>[2x]MSLPMLQVALDNQTM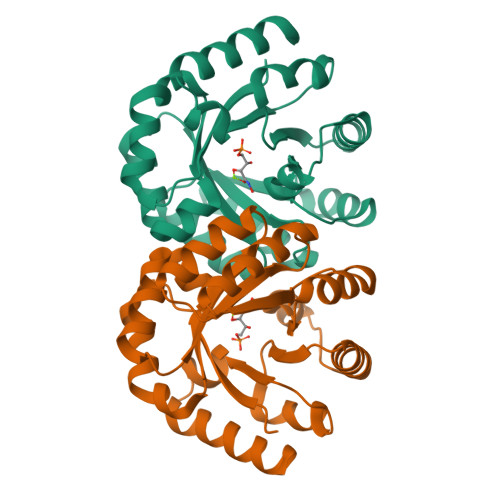DSAYETTRLIAEEVDIIEVGTILCVGEGVRAVRDLKALYPHKIVLADAKIADAGKILSRMCFEANADWVTVICCADINTAKGALDVAKEFNGDVQIQLTGYWTWEQAQQWRDAGIGQVVYHRSRDAQAAGVAWGEADITAIKRLSDMGFKVTVTGGLALEDLPLFKGIPIHVFIAGRSIRDAASPVEAARQFKRSIAELWG> MIGRLRGIIIEKQPPLVLIEVGGVGYEVHMPMTCFYELPEAGQEAIVFTHFVVREDAQLLYGF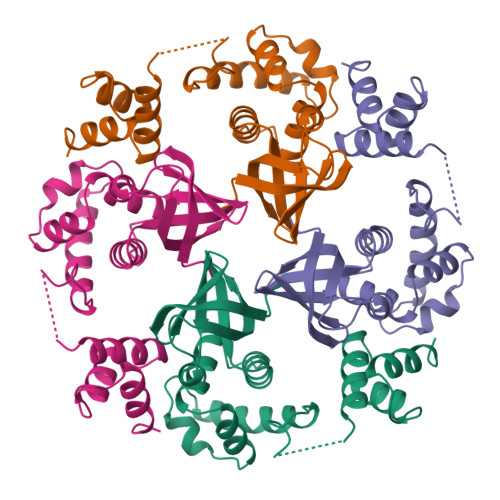NNKQERTLFKELIKTNGVGPKLALAILSGMSAQQFVNAVEREEVGALVKLPGIGKKTAERLIVEMKDRFKGLHGDLFTPAADLVLTSPASPATDDAEQEAVARLVALGYKPQEASRMVSKIARPDASSETLIREALRAAL>[2x]MGSDKIHHHHHHENLYFQGMWEIYDAMINGIPEDFLVDELVCGTTHSVIRSGNGVGLGPNRPFETRMPMLTQNLLGLPLRVAAGCVKSWNYVEASIGLAAINAYYNNPQVAREHGVIFSDAKRVEDRMNDPFIMSQN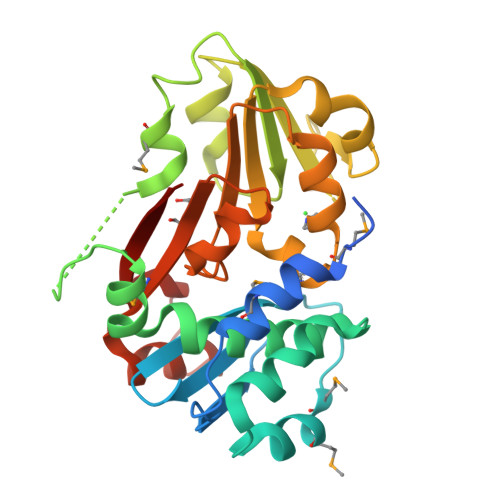EVKGKKVGVVGHFPHLESLLEPICDLSILEWSPEEGDYPLPASEFILPECDYVYITCASVVDKTLPRLLELSRNARRITLVGPGTPLAPVLFEHGLQELSGFMVKDNARAFRIVAGAEKVKIYSAGQKVTIKK>[2x]MRGSHHHHHHGSVTCTGCVDLDELSFEKTVERFPYSVVKFDIASPYGEKHEAFTAFSKS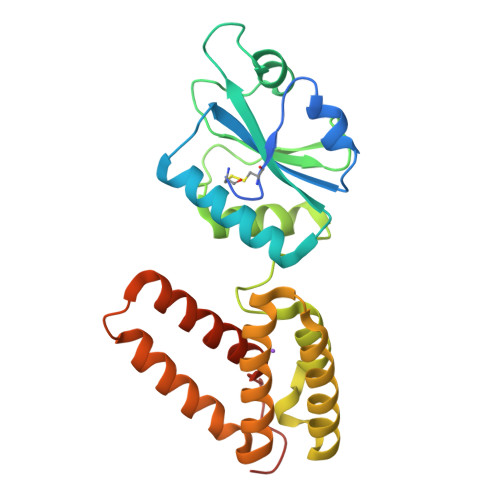AHKATKDLLIATVGVKDYGELENKALGDRYKVDDKNFPSIFLFKGNADEYVQLPSHVDVTLDNLKAFVSANTPLYIGRDGCIKEFNEVLKNYANIPDAEQLKLIEKLQAKQEQLTDPEQQQNARAYLIYMRKIHEVGYDFLEEETKRLLRLKAGKVTEAKKEELLRKLNILEVFRVHKVTKTAPEKEEL[(1~{R})-1-[1-(phenylmethyl)-1,2,3,4-tetrazol-5-yl]butyl]diazane 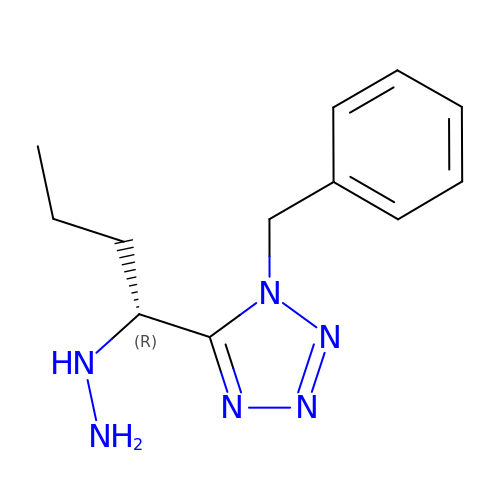| C12 H18 N6 | RXFMIKHNJVMPGC-LLVKDONJSA-N Recently, we demonstrated that cmo5U modification requires the previously unknown metabolite carboxy-S-adenosine-L-methionine (Cx-SAM), which is generated by the CmoA-catalyzed conversion of prephenate and SAM to yield Cx-SAM and phenylpyruvate. Cx-SAM is subsequently utilized in the CmoB-catalyzed carboxymethylation of ho5U-containing tRNAs to yield the mature cmo5U-modified tRNAs, with no involvement of a mo5U intermediate. As predicted from sequence considerations, CmoB is composed of a Rossmann fold, coupled to a substrate-specific N-terminal domain of ∼100 residues that is unique to CmoB. Our biochemical, genetic and structural data demonstrate that the primary in vivo function of CmoB is as a carboxymethyl transferase in the biosynthesis of cmo5U-modified tRNAs.

Cx-SAM bound CmoB structures were determined in two crystal forms, resulting in 10 independent copies of the complex (two tetramers in one crystal form, and one dimer in the other), while the apo structure contains a single dimer in the asymmetric unit. Difference Fourier syntheses calculated after initial rounds of refinement, without the inclusion of ligand, exhibited features consistent with the binding of Cx-SAM in the catalytic site. Continued refinement and modeling indicated that Cx-SAM is present at full occupancy and demonstrated similar atomic interactions in all 10 independent catalytic sites in both liganded structures. The side chains of Lys-91, Tyr-200 and Arg-315 interact with the carboxyl group of the S-carboxymethyl moiety of the Cx-SAM ligand. Three additional conserved residues within the CmoB family recognize the amino acid moiety of the ligand: the side chain of Lys-110 (815/818) forms polar interactions with the α-carboxy group, while the backbone carbonyl oxygen atoms of Gly-130 (817/818; the presence of a bulkier side chain would likely interfere with ligand binding) and Met-196 (606/818, where other instances are leucine) interact with the α-amino group of Cx-SAM. The side chain of Glu-182 (96% conservation) forms polar interactions with N6 of the adenine moiety and the side chain of Asp-152 (∼97% conserved in CmoB orthologs, and highly conserved in all members for SAM-dependent methyltransferase superfamily) interacts with the 2′- and 3′-hydroxyls. In contrast, backbone oxygen atoms of Met-196 and Gly-197 of CmoB form potential carbon–oxygen hydrogen bonding interactions with the other two methylene groups adjacent to the sulfonium center of Cx-SAM; these interactions are absent in the CmoA structure. Within the catalytic site of CmoB, Cx-SAM is highly exposed to the bulk solvent, whereas in CmoA it is substantially more buried. In all subunits in both Cx-SAM bound structures, a feature modeled as a phosphate ion is present between two basic residues, Arg-202 and His-208 (98.3 and 67.1% conservation, respectively), with one of the presumed sulfate ions from the crystallization media present at a similar position in the apo structure.

>[8x]MIDFGNFYSLIAKNHLSHWLETLPAQIANWQREQQHGLFKQWSNAVEFLPEIKPYRLDLLHSVTAESEEPLSAGQIKRIETLMRNLMPWRKGPFSLYGVNIDTEWRSDWKWDRVLPHLSDLTGRTILDVGCGSGYHMWRMIGAGAHLAVGIDPTQLFLCQFEAVRKLLGNDQRAHLLPLGIEQLPALKAFDTVFSMGVLYHRRSPLEHLWQLKDQLVNEGELVLETLVIDGDENTVLVPGDRYAQMRNVYFIPSALALKNWLKKCGFVDIRIADVSVTTTEEQRRTEWMVTESLADFLDPHDPGKTVEGYPAPKRAVLIARKP> GAMGLPGAEEAPVRVALRVRPLLPKELLHGHQSCLQVEPGLGRVTLGRDRHFGFHVVLAE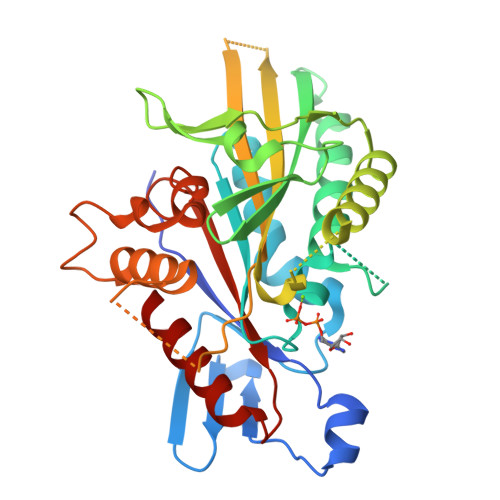DAGQEAVYQACVQPLLEAFFEGFNATVFAYGQTGSGKTYTMGEASVASLLEDEQGIVPRAMAEAFKLIDENDLLDCLVHVSYLEVYKEEFRDLLEVGTASRDIQLREDERGNVVLCGVKEVDVEGLDEVLSLLEMGNAARHTGATHLNHLSSRSHTVFTVTLEQRGRAPSRLPRPAPGQLLVSKFHFVDLAGSERVLKTGSTGERLKESIQINSSLLALGNVISALGDPQRRGSHIPYRDSKITRILKDSLGGNAKTVMIACVSPSSSDFDETLNTLNYASRAQ> GGSHDCAKVDLENAELRRKLIRTKRAFEDTYEKLRMANKAKAQVEKDIKNQILKTHNVLRNVRSNMEN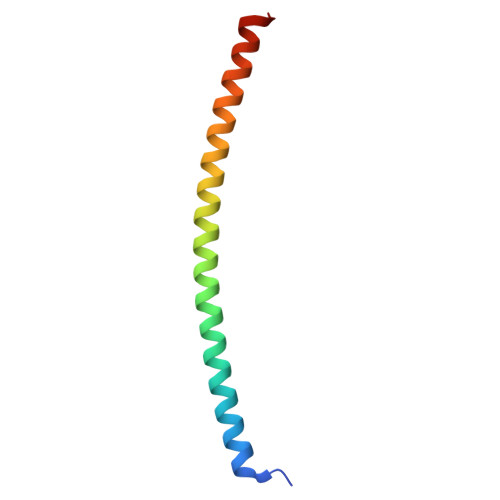EL> MVQPFAWQV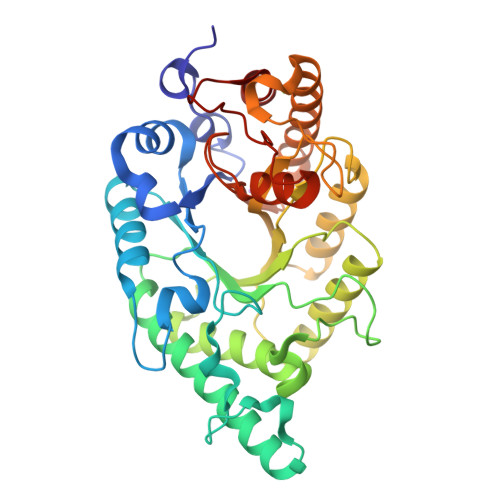ASLADRYEESFDIGAAVEPHQLNGRQGKVLKHHYNSIVAENAMKPISLQPEEGVFTWDGADAIVEFARKNNMNLRFHTLVWHNQVPDWFFLDEEGNPMVEETNEAKRQANKELLLERLETHIKTVVERYKDDVTAWDVVNEVVDDGTPNERGLRESVWYQITGDEYIRVAFETARKYAGEDAKLFINDYNTEVTPKRDHLYNLVQDLLADGVPIDGVGHQAHIQIDWPTIDEIRTSMEMFAGLGLDNQVTELDVSLYGWPPRPAFPTYDAIPQERFQAQADRYNQLFELYEELDADLSSVTFWGIADNHTWLDDRAREYNDGVGKDAPFVFDPNARVKPAFWRIID>GSHMNINKQSPIPIYYQIMEQLKTQIKNGELQPDMPLPSEREYAEQFGISRMTVRQALSNLVNEGLLYRLKGRGTFVSKPKMEQALQGLTSFTEDMKSRGMTPGSRLIDYQLIDSTEELAAILGCGHPSSIHKITRVRLANDIPMAIESSHIPFELAGELNESHFQSSIYDHIERYNSIPISRAKQELEPSAATTEEANILGIQKGAPVLLIKRTTYLQNGTAFEHAKSVYRGDRYTFVHYMDRLS[2x]

NagR, formerly termed YvoA, has been identified as a repressor protein from Bacillus subtilis that regulates genes involved in N-acetylglucosamine (GlcNAc) utilization. NagR acts as a negative transcriptional regulator, and binding of effector-free NagR to specific DNA operator sites blocks gene transcription. With more than 49000 deposited sequences, the GntR family of regulators (gluconate-operon repressor, Pfam family: PF00392) represents one of the largest groups of bacterial metabolite-responsive transcription factors. Their tertiary structure can be subdivided in almost all cases into two distinct domains: an N-terminal DNA-binding winged-helix-turn-helix (wHTH) domain and a C-terminal small-molecule effector-binding and oligomerization domain. In NagR and the entire GntR/HutC subfamily the C-terminal effector-binding domain adopts a so-called UTRA domain fold (Pfam family: PF07702) that is structurally homologous to the enzyme chorismate lyase.

To gain insight into DNA binding in the GntR/HutC subfamily of repressors, we determined the crystal structure of full-length NagR in complex with an idealized palindromic operator dre-site at 2.9 Å resolution. The asymmetric unit contains one NagR dimer in complex with a 19 bp fragment of dsDNA. Electron density is missing for several segments in the effector-binding domain as well for the peptide segment that interconnects the effector-binding domain and the DBD in each chain A and B of homodimeric NagR. In detail, helices αE3, αE4 and αE5 are not formed in chain A, while chain B lacks most parts of helix αE3 as well as the N-terminal ends of helices αE2 and αE5. Regarding the interdomain linker, residues 79 to 83 and residues 81 to 85 are missing in chain A and B, respectively. Apart from the striking absence of beta-strand β*, which occurs in the interdomain linker region of the GlcN-6-P and GlcNAc-6-P-bound state of NagR, DNA-bound NagR features a highly similar topology consisting of nine α-helices and nine β-strands. In the DNA-bound complex, the DBDs of NagR are pointing downward in direction of the very C-terminal strand βE7, which is in agreement with our previously proposed NagR DNA-binding model derived from YydK. Surprisingly, the orientation of the two-fold symmetry axis that relates the two effector-binding domains in NagR does not coincide with the two-fold axis that relates the two DBDs bound to the 19 bp palindromic DNA fragment since a crossing angle of 6.5° can be observed between the two local symmetry axes. Thus it appears that in the DNA-bound and ligand-free structure of NagR not only secondary structure elements in the effector-binding domain are considerably less well defined but that also the DBDs are more flexibly attached to the effector-binding domain than in GlcN-6-P- and GlcNAc-6-P-bound NagR.>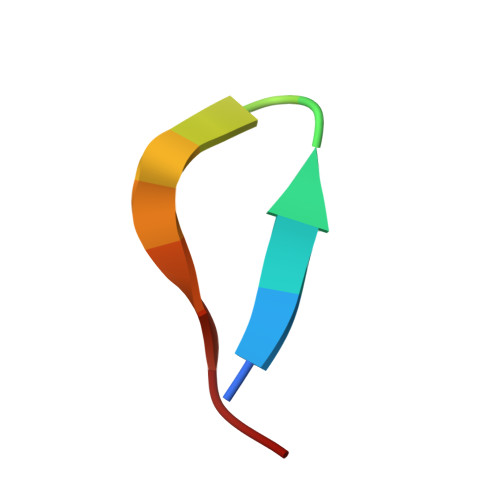 WRYYESSLLPYPD> MEETRPIDGLTDEDIREILTRYKKIALVGASPKPERDANIVMKYLLE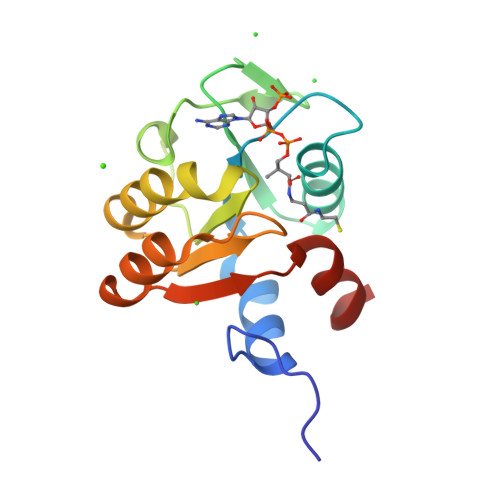HGYDVYPVNPKYEEVLGRKCYPSVLDIPDKIEVVDLFVKPKLTMEYVEQAIKKGAKVVWFQYNTYNREASKKADEAGLIIVANRCMMREHERLLGEK>GSYDYLFKVVLIGDSGVGKSNLLS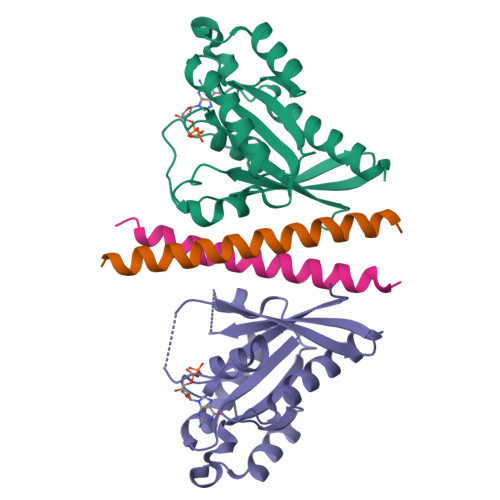RFTRNEFNLESKSTIGVEFATRSIQVDGKTIKAQIWDTAGQERYRAITSAYYRGAVGALLVYDIAKHLTYENVERWLKELRDHADSNIVIMLVGNKSDLRHLRAVPTDEARAFAEKNNLSFIETSALDSTNVEEAFKNILTEIYRIVSQKQIADRAAHDESPGNNVVDISVPPTTD[2x];>GSKDAELQEREYHLKELREQLAKQTVAIAELTEELQSKCIQLNKLQ[2x]> SNAVRLRASEIMNRTLDLQIIMDDLLNLLLKEFKLDLAVIRLVDEKGVLRVRSYSGKGIAGIAGKDWEPEIETYIGEAFLSNRLQFVNDTQYMTKPLTRELMQKEGIKSFAHIPISRKGEPPFGILSVFSRTIVGLFNEPFLNLLESLAGQLA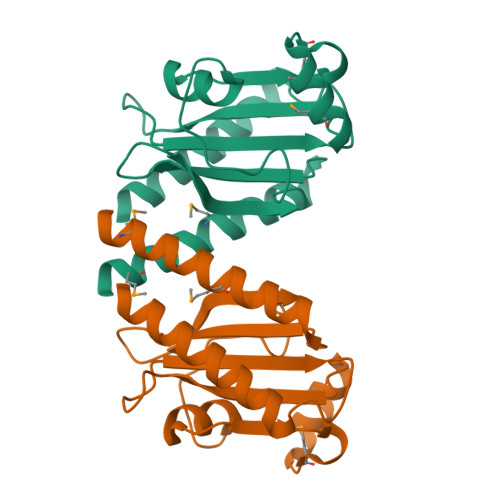QAVKIVTEMEAKEREREEKERILLENAR>[4x]QDFAELQGKWYTIVIAADNLEKIEEGGPLRFYFRHIDCYKNCSEMEITFYVITNNQCSKTTVIGYLKGNGTYETQFEGNNIFQPLYITSDKIFFTNKNMDRAGQETNM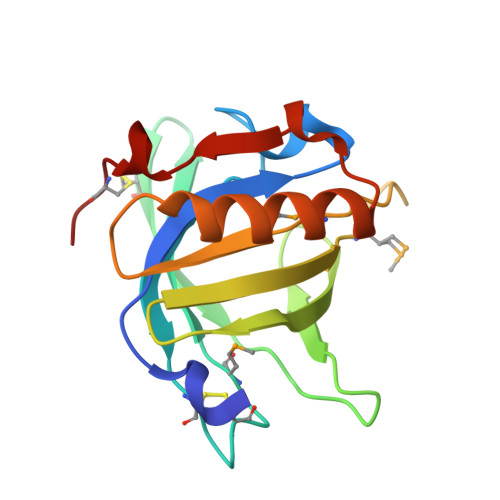IVVAGKGNALTPEENEILVQFAHEKKIPVENILNILATDTCPE>[2x]MGQGPELHLASQFVNEACRALVFGGCVEKSSVSRNPEVPFESSAYRISASARGKELRLILSPLPGAQPQQEPLALVFRFGMSGSFQLVPREELPRHAHLRFYTAPPGPRLALCFVDIRRFGRWDLGGKWQPGRGPCVLQEYQQFRENVLRNLADKAFDRPICEALLDQRFFNGIGNYLRAEILYRLKIPPFEKARSVLEALQQHRPSPELTLSQKIRTKLQNPDLLELCHSVPKEVVQLGGKGYGSESGEEDFAAFRAWLRCYGMPGMSSLQDRHGRTIWFQGDPGPLAPKGRKS

Human endonuclease VIII-like 1 (hNEIL1) is a bifunctional DNA glycosylase of the Fpg/Nei family, which catalyzes the removal of damaged bases and subsequent incision of the newly generated abasic sites. Unlike traditional enzymes which are commonly referred to as highly specific biocatalysts, one special feature for hNEIL1 is its unique capability to recognize a wide range of substrates, including formamidopyrimidines, hydantoin lesions, oxidized, and dihydro-modified pyrimidine bases, derived from all four canonical bases. Here, by integrating structural, computational, and biochemical investigations, we show that hNEIL1 uses a triage mechanism to achieve broad specificity and reduce futile repair of normal bases. This mechanism involves two mutually competing interaction states: an activated state that commits catalysis and BER, and a quarantine state that temporarily separates and prevents the flipped base from catalysis via auto-inhibition.

While we also crystallized the complex structures for more lesions in this study, we were unable to obtain intact substrates in the active site of hNEIL1, presumably due to the residual glycosylase activity. Hence, we introduced an extra E3Q mutation to the truncated hNEIL1(C∆95 P2G) (see the “Methods” section) and succeeded in the determination of complex structures containing 5-hydroxyuracil (5-OHU), spiroiminodihydantoin 1 (Sp1), (S)-guanidinohydentoin (Gh), dihydrothymine (DHT) and dihydrouracil (DHU), respectively. Despite the very different chemical structures of these substrates, they are recognized similarly by hNEIL1. The damaged bases are fully extruded from the DNA helix and inserted into a relatively loose binding pocket, which allows the accommodation of substrates with varying sizes and shapes. One edge of the flipped base points towards the protein and forms close contact with the side chain of K242. Noteworthy, across all these structures, we observed an unusually short distance (~3.0 Å) between an outwards heterocyclic nitrogen atom of the nucleobases and the terminal nitrogen atom of residue 242. Based on the similar overall conformation and detailed atomic interactions, we conclude that such a tautomerization-dependent mechanism may be a general strategy for hNEIL1 to recognize not only Tg but also 5-OHU, Sp1, Gh, DHT, and DHU. Oxidized substrates of hNEIL1 are often bulky and contain non-planar structures; this disrupted aromaticity is expected to diminish the π–π stacking with Tyr244 and hence destabilize the quarantine state. Moreover, it is expected that the bases with less solvent interactions (e.g. DHU) would favor the formation of a stable quarantine state compared with the hydrophilic bases (Sp1, 5-OHU, Gh, and Tg).> MAEQDPKELVGLGAKSYKEKDFTQAKKYFEKACDLKENSGCFNLGVLYYQGQGVEKNLKKAASFYAKACDLNYSNGCHLLGNLYYSG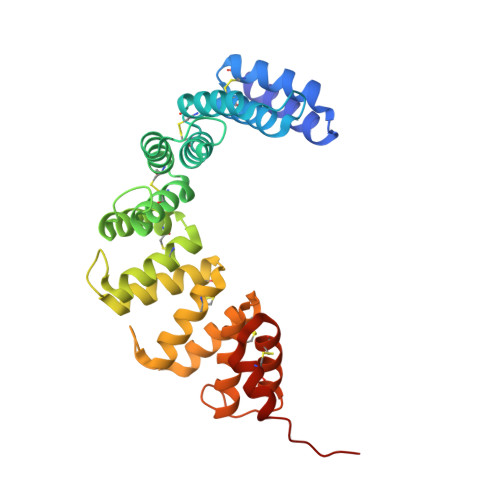QGVSQNTNKALQYYSKACDLKYAEGCASLGGIYHDGKVVTRDFKKAVEYFTKACDLNDGDGCTILGSLYDAGRGTPKDLKKALASYDKACDLKDSPGCFNAGNMYHHGEGATKNFKEALARYSKACELENGGGCFNLGAMQYNGEGVTRNEKQAIENFKKGCKLGAKGACDILKQLKIKVHHHHHH Diacylglycerol (DAG) is a versatile lipid whose 1,2-sn-stereoisomer serves both as second messenger in signal transduction pathways that control vital cellular processes, and as metabolic precursor for downstream signaling lipids such as phosphatidic acid. Effector proteins translocate to available DAG pools in the membranes by using conserved homology 1 (C1) domains as DAG-sensing modules. PKCs define a central DAG-sensing node in intracellular phosphoinositide signaling pathways that regulate cell growth, differentiation, apoptosis, and motility. Herein, we report the high-resolution crystal structures of a C1 domain (C1B from PKCδ) complexed to DAG and to each of four potent PKC agonists that produce different biological readouts and that command intense therapeutic interest.

AJH-836 is a high-affinity synthetic DAG lactone with considerable promise as an isoenzyme-specific PKC agonist. The DHPC-protein interactions involve hydrogen bonds, both direct and water-mediated, as well as hydrophobic contacts. The structure of the AJH-836, where one protein chain has a bound ligand and the other ligand-free chain interacts peripherally with DHPC, highlights the versatility of interactions that Trp252 at the “DAG-toggling” position can form with lipids. In e, one protein chain is ligand-free (color-coded green) and has three DHPC molecules, labeled 1 through 3 that cap the membrane-binding loop region. f The versatility of potential Trp252-lipid interactions, exemplified by the Trp252 sidechain from the ligand-free C1Bδ monomer (e green). In addition to non-polar contacts with the hydrophobic lipid moieties, the Trp sidechains can engage in H-bonding, cation–π, and CH–π interactions. The structures reveal that all four ligands bind to the same C1Bδ site as DAG. AJH-836 is the only ligand of the four with no additional ligand-protein hydrogen bonds compared to DAG. In the lactone complex, a combination of the E isomer and its “sn-1” binding mode affords a favorable arrangement of bulky R1 and R2 groups within the hydrophobic rim of C1Bδ. This configuration likely constitutes the structural basis for why AJH-836 displays its marked selectivity for novel versus conventional PKC isoforms.

>MPHRFKVYNYMSPTFCDHCGSLLWGLVKQGLKCEDCGMNVHHKCREKVANLCG[2x]> MQQLNENKIIKLLRDNIPKLQLIYLFGSYSQGTQHRNSEIEIAVLAADTLDNIARWELAQKLASALDSDVDLVDLRSASTVLCQQVVTQGKQLWGTQQDDELFAVKTISMYQHLQAERQAIIDDVMANT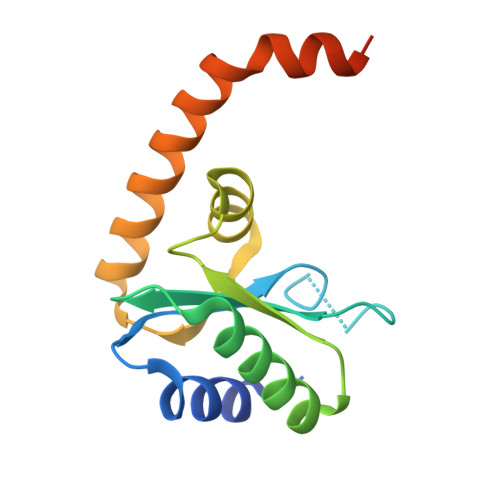AAKAHRGESL> MRLAYVKNHEIYGEKLLGLTLRERIEKTLQRAGFDVRFFDELSLEEAEDYLIILEPVLILERDLLLEGRKILVSDGFTVGYFFGGDFRTVFDGNLQSSIEKYLSLNNLESYEIWAIKLSNDNLKTAEKLLLSSLIGSRGLFAAIFLPIARLLADWGVSPDAVTVVGTLGVMAGALIFYPMGQLFWGT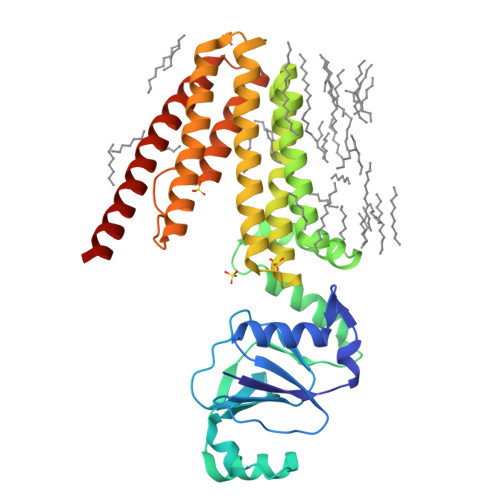VVITVFVFSDIIDGLMARLLFREGPWGAFLDSYLDRVGDSSVFTGIVIWFFLGGANPTIAILALICLVLSSLVSYSKARAEGLGLTANVGIAERSERLVVVLVATGLVGLGIPSWVLLVVLIVLAIASVVTIFQRVLTVREQAKAWTAS>[2x]MGHHHHHHHHHHSSGHIDDDDKHMPAHASPFNAPSSASRAGAARLGTSRRFAPFVLAALAILMGAMSVVALCVGAYRIPLAEAWAALSGDPAAQQARAVLLDIRAPRVVLALLVGGGFGATG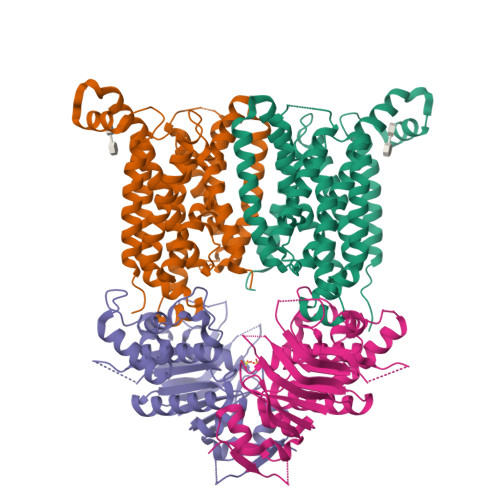AAMQALFRNPLADPGLVGVSSGAALGATTLIVLGPALFAAHASAAALPVAAFAGGLAVAALVYRLAASRGRLALPLLLLAGIAINALVGAAIGLLTFVADDAQLRSLTFWSLGSLGGAQWPTLAAVAPCVALGGVLLVRERDALNALQLGETEALHLGVPVQRLKRRVLVAVALAVGALVSCAGIIGFIGLVAPHCVRLACGPDQRIVLPGAALLGALLTLAADLAARTVAAPADIPLGVLTALLGAPFFLALLWKNRGALGG;>MLTAHHLDVARRHGTILRDLSLSIEPGRVTALLGRNGAGKSTLLKTFAGELTGSVAPHGVRVTGDVTLNGEPLARIDAPRLACLRAVLPQAAQPAFPFSVDEIVLLGRYPHARRSGATSHRDRDIAWRALERAGADALVGRDVTTLSGGELARVQFARVLAQLWPDHDTTEPGPRYLLLDEPTAALDLAHQHRLLDTVRAVAREWQLGVLAIVHDPNLAARHADAIAMLADGTIVAHGAPRDVMTPAHIAQCYGFAVKMVETGDGTPPVMVPA[2x]> GSELTPDQQTLLHFIMDSYNKQRMPQEITNKILKEEFSAEENFLILTEMATNHVQVLVEFTKKLPGFQTLDHEDQIALLKGSAVEAMFLRSAEIFNKKLPSGHSDLLEERIRNSGISDEYITPMFSFYKSIGELKMTQEEYALLT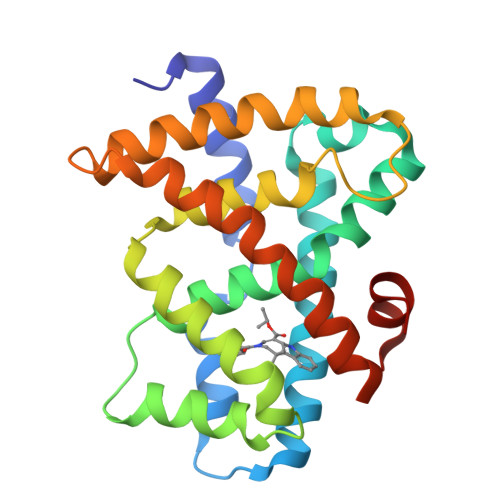AIVILSPDRQYIKDREAVEKLQEPLLDVLQKLCKIHQPENPQHFACLLGRLTELRTFNHHHAEMLMSWRVNDHKFTPLLCEIWDVQ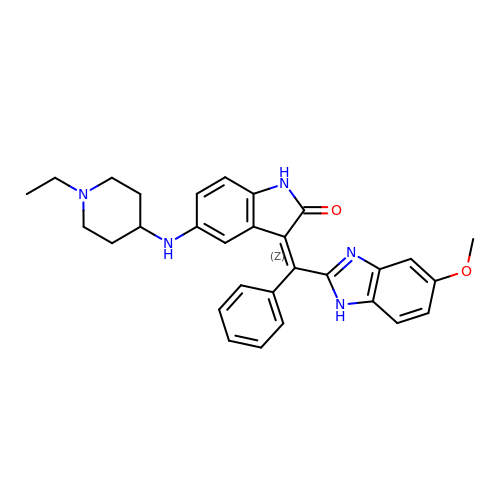(3Z)-5-[(1-ethylpiperidin-4-yl)amino]-3-[(5-methoxy-1H-benzimidazol-2-yl)(phenyl)methylidene]-1,3-dihydro-2H-indol-2-one | C30 H31 N5 O2 | LETIJBVXDGOQFG-DQSJHHFOSA-N> QSLVADVGDDHHAWHRLLDQALNQRRFELFFQPVVAAQDTQLVLHYKVLSRLLDEQGQTIPAGRFLPWLERFGWTARLDRLMLERVLEQMAGHEESLALNLSSATLADPQALNKVFEILRAHSNLGARLTLEIGEEQLPEQAVLEQLTRRLRELGFSLSLQRFGGRFSMIGNLARLGLAYLKIDGSYIRAIDQESDKRLFIEAIQRAAHSIDLPLIAERVETEGELSVIREMGLYGVQGQLFGEPKPWG

Here, we elucidated the molecular mechanism underlying the function and regulation of P. fluorescens LapD, a transmembrane receptor essential for biofilm formation in this strain. As c-di-GMP levels change LapD switches between two states: the dinucleotide-unbound off state that retards stable biofilm formation by facilitating the secretion of the cell surface adhesin LapA, and the c-di-GMP-bound on state that supports cell adhesion by preventing the release of LapA from the outer membrane. Binding of c-di-GMP to the LapD EAL domain is relayed to the periplasmic output domain through an inside-out signaling mechanism that utilizes a juxtamembrane HAMP domain, a relay module often found in bacterial transmembrane receptors. Here, we present three crystal structures of LapD from P. fluorescens that provide models for the c-di-GMP-unbound cytoplasmic domain lacking only the HAMP domain, a c-di-GMP-bound EAL domain dimer, and the periplasmic domain.

The crystal structure of LapDEAL bound to c-di-GMP (residues 399–648; LapDEAL•c-di-GMP) was solved by molecular replacement using the EAL domain from apo-LapDdual as the search model. We obtained crystals in two independent conditions, yielding two different crystal forms (space group C2221, two molecules per asymmetric unit; and space group P6522, one molecule per asymmetric unit). While the majority of the crystal packing contacts were different, both crystal forms maintained a common dimer of EAL domains, and the resulting structures superimposed almost perfectly (rmsd of 0.6 Å over all atoms). c-di-GMP binding did not alter the overall conformation of the EAL domain observed in the apo-LapDdual structure (rmsd of 0.6 Å over all atoms), consistent with the lack of major conformational changes upon dinucleotide binding to the EAL domains of YkuI, TDB1265, and FimX. The most notable conformational change in LapDEAL upon c-di-GMP binding occurs in the switch loop. Dinucleotide binding and the absence of the S helix in the isolated EAL domain allow the loop to restructure, resulting in the switching of the conserved phenylalanine residue F566. In contrast, the switch loop adopts a conformation in the c-di-GMP-bound structure positioning F566 so that it can participate in homodimerization. The symmetric LapDEAL domain dimer is reminiscent of the oligomeric state in active EAL domain–containing phosphodiesterases, such as in P. aeruginosa SadR/RocR, Bacillus subtilis YkuI, Thiobacillus denitrificans TDB1265, and the BLUF domain–regulated photoreceptor BlrP1 from Klebsiella pneumoniae, where dimerization is involved in positioning an aspartate residue that in the active protein coordinates a cation for efficient catalysis. Most importantly, dimerization of the c-di-GMP-bound EAL domains is incompatible with the conformation observed in the crystals of apo-LapDdual.>MSTPKIIYTLTDEAPALATYSLLPIIKAFTGSSGIAVETRDISLAGRLIATFPEYLTDTQKISDDLAELGKLATTPDANIIKLPNISASVPQLKAAIKELQQQGYKLPDYPEEPKTDTEKDVKARYDKIKGSAVNPVLREGNSDRRAPLSVKNYARKHPHKMGAWSADSKSHVAHMDNGDFYGSEKAALIGAPGSVKIELIAKDGSSTVLKAKTSVQAGEIIDSSVMSKNALRNFIAAEIEDAKKQGVLLSVHLKATMMKVSDPIMFGQIVSEFYKDALTKHAEVLKQIGFDVNNGIGDLYARIKTLPEAKQKEIEADIQAVYAQRPQLAMVNSDKGITNLHVPSDVIVDASMPAMIRDSGKMWGPDGKLHDTKAVIPDRCYAGVYQVVIEDCKQHGAFDPTTMGSVPNVGLMAQKAEEYGSHDKTFQIPADGVVRVTDESGKLLLEQSVEAGDIWRMCQAKDAPIQDWVKLAVNRARATNTPAVFWLDPARAHDAQVIAKVERYLKDYDTSGLDIRILSPVEATRFSLARIREGKDTISVTGNVLRDYLTDLFPIMELGTSAKMLSIVPL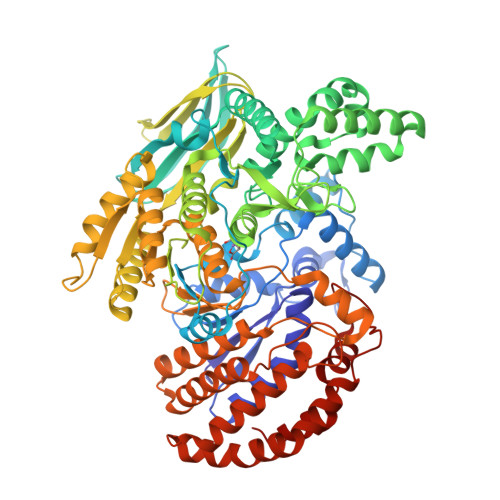MSGGGLFETGAGGSAPKHVQQFLEEGYLRWDSLGEFLALAASLEHLGNAYKNPKALVLASTLDQATGKILDNNKSPARKVGEIDNRGSHFYLALYWAQALAAQTEDKELQAQFTGIAKALTDNETKIVGELAAAQGKPVDIAGYYHPNTDLTSKAMRPSATFNAALAPLA[4x]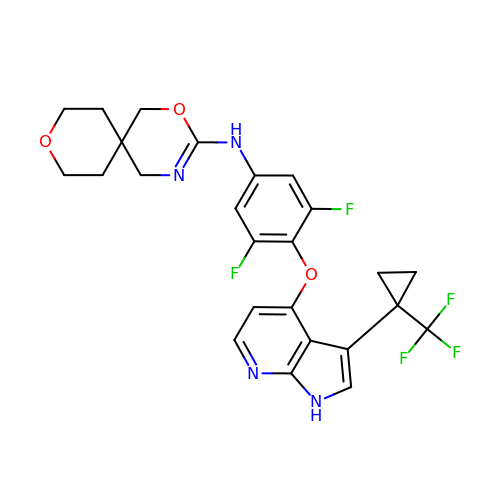~{N}-[3,5-bis(fluoranyl)-4-[[3-[1-(trifluoromethyl)cyclopropyl]-1~{H}-pyrrolo[2,3-b]pyridin-4-yl]oxy]phenyl]-2,9-dioxa-4-azaspiro[5.5]undec-3-en-3-amine | C25 H23 F5 N4 O3 | FXMIIWBGTCDJJQ-UHFFFAOYSA-N> MSRFQSLLCFVLVSLAAVANAAIGPVADLTLTNAAVSPDGFSREAVVVNGVTPAPLISGQKGDRFQLNVIDNLTNHTMLKTTSIHWHGFFQHG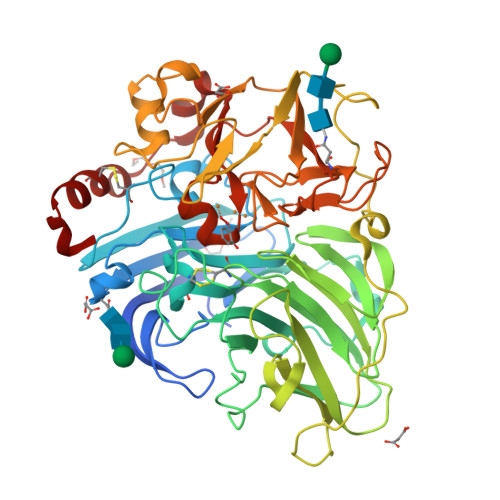TNWADGPAFVNQCPIASGHSFLYDFQVPDQAGTFWYHSHLSTQYCDGLRGPFVVYDPNDPQASLYDIDNDDTVITLADWYHVAAKLGPRFPPGSDATLINGLGRSPGTTAADLAVIKVTQGKRYRFRLVSLSCDPNHTFSIDGHTMTIIEADSVNTQPLEVDSIQIFAAQRYSFVLDASQPVDNYWIRANPSFGNTGFAGGINSAILRYLGAPEIEPTTTQTTPTKPLTEVDLHPLTPMAVPGRPEPGGVDKPLNMVFNFNGTNFFINNHSFVPPSVPVLLQILSGAQAAQDLVPEGSVYVLPSNSSIEISFPATVNAPGAPHPFHLHGHTFAVVRSAGSSEYNYDNPIFRDVVSTGTPGDNVTIRFQTANPGPWFLHCHIDFHLDAGFAVVMAEDTPDTTAANPVPQAWSDLCPIYDALDPSDL>MAHHHHHHMNLRAAGPGWLFCPADRPERF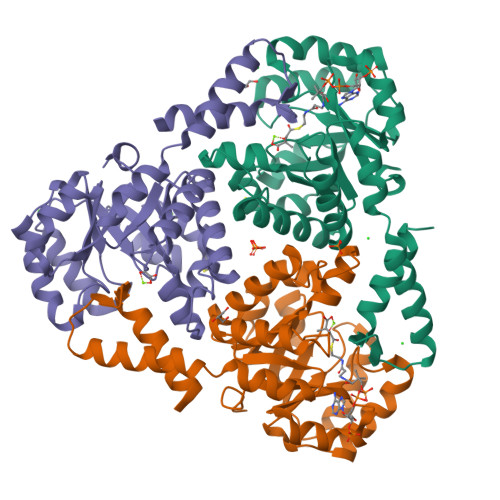AKAAAAADVVILDLEDGVAEAQKPAARNALRDTPLDPERTVVRINAGGTADQARDLEALAGTAYTTVMLPKAESAAQVIELAPRDVIALVETARGAVCAAEIAAADPTVGMMWGAEDLIATLGGSSSRRADGAYRDVARHVRSTILLAASAFGRLALDAVHLDILDVEGLQEEARDAAAVGFDVTVCIHPSQIPVVRKAYRPSHEKLAWARRVLAASRSERGAFAFEGQMVDSPVLTHAETMLRRAGEATSE[3x]> MHHHHHHKNITNASILSIVYKDDDLIDLSRYGAEIYNGDKVYYNSIDKNQIRLINLESSTIEVILKKAIVYNSMYENFSTSFWIRIPKYFNSISLNNEYTIINCMENNSGWKVSLNYGEIIWTFQDTQEIKQRVVFKYSQMINISDYINRWIFVTITNNRITKSKIYINGRLID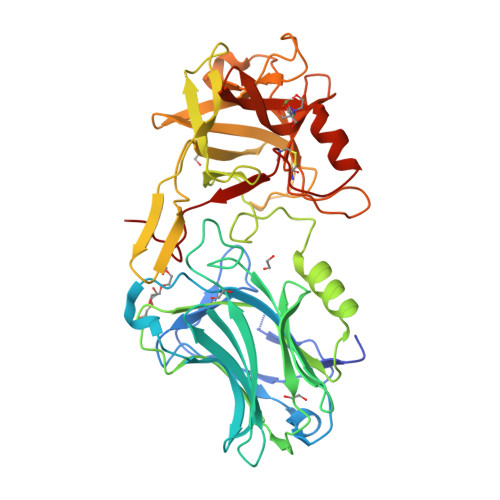QKPISNLGNIHASNKIMFKLDGCRDPHRYIVIKYFNLFDKELSEKEIKDLYDNQSNSGILKDFWGDYLQYDKSYYMLNLYDPNKYVDVNNVGIRGYMYLKGPRDNVMTTNIYLNSSLYMGTKFIIKKYASGNKDNIVRNNDRVYINVVVKNKEYRLATNASQAGVEKILSALEIPDVGNLSQVVVMKSKNDQGITNKCKMNLQDNNGNDIGFIGFHQFNNIAKLVASNWYNRQIERSSRTLGCSWEFIPVDDGWRERPL Two new modified Bacillus thuringiensis (Bt) proteins, Cry1Da_7 and Cry1B.868, with activity against fall armyworms (FAW), Spodoptera frugiperda (J.E. Smith), were evaluated for their potential to bind new insect receptors compared to proteins currently deployed as plant-incorporated protectants (PIPs) in row crops. Results from resistant insect bioassays, disabled insecticidal protein (DIP) bioassays, and cell-based assays using insect cells expressing individual receptors demonstrate that receptor utilizations of the newly modified Cry1Da_7 and Cry1B.868 proteins are distinct from each other and from those of commercially available Bt proteins such as Cry1F, Cry1A.105, Cry2Ab, and Vip3A. Accordingly, these two proteins target different insect proteins in FAW midgut cells and when pyramided together should provide durability in the field against this economically important pest. Taken together, these results support the conclusion that Cry1Da_7 and Cry1B.868 are effective insecticidal proteins against FAW that have the same pore-forming mode of action as other three-domain Bt proteins but bind to different receptors, suggesting that they would control resistance and increase product durability.

Cry1B.868 was developed using chimeragenesis, similar to the method used to develop the Cry1A.105 protein, a familiar protein that has been deployed commercially as Bt maize protected against FAW. Cry1B.868 exerted mortality and developmental delay on FAW (and other lepidopteran insects [not shown]) at concentrations between 100 and 34,500 ng/cm2. Its MIC50 of 430 ng/cm2 against FAW using gradient-purified protein suggested an 8-fold improvement in specific activity toward this insect compared to the parental Cry1Be2 protein. There was no detectable difference in insect responses between the Cry1Fa-SS and Cry1Fa-RR colonies for both Cry1Da_7 and Cry1B.868, suggesting that the Cry1F-resistant colony was not cross-resistant to either Cry1Da_7 or Cry1B.868. Cry1B.868 was also highly toxic to the FAW colonies, with LC50 values of 262 ng/cm2 against the Vip3A-SS colony and 43 ng/cm2 against the Vip3A-RR colony, indicating a lack of cross-resistance. Interestingly, the Vip3A-resistant colony was significantly more sensitive to Cry1B.868 than the Vip3A-susceptible colony was; the data suggest that this difference is unrelated to the Vip3A resistance allele, and it is likely due to slight genetic background differences between the susceptible and resistant colonies. Cry1B.868 at 50 μg/ml elicited robust membrane permeabilization in Sf9 cells expressing Sf.ABCb1, while only a background signal was observed when this receptor was not expressed. These results indicate that SfABCb1 and Cry1B.868 are a functional receptor-toxin pair.

> IEDSLCIAEGNNIDPFVSASTVQTGINIAGRILGVLGVPFAGQIASFYSFLVGELWPRGRDPWEIFLEHVEQLIRQQVTENTRDTALARLQGLGNSFRAYQQSLEDWLENRDDARTRSVLYTQYINLELDFLDAMPLFAIRNQEVPLLMVYAQAANLHLLLLRDASLFGSEFGLTSQEIQRYYERQVEKTREYSDYCARWYNTGLNNLRGTNAESWLRYNQFRRDLTLGVLDLVALFPSYDTRVYPMNTSAQLTREIYTDPIGRTNAPSGFASTNWFNNNAPSFSAIEAAVIRPPHLLDFPEQLTIFSVLSRWSNTQYMNYWVGHRLESRTIRGSLSTSTHGNTNTSINPVTLQFTSRDVYRTESFAGINILLTTPVNGVPWARFNWRNPLNSLRGSLLYTIGYTGVGTQLFDSETELPPETTERPNYESYSHRLSNIRLISGNTLRAPVYSWTHRSADRTNTISSDSITQIPLVKAHTLQSGTTVVKGPGFTGGDILRRTSGGPFAFSNVNLDFNLSQRYRARIRYASTTNLRIYVTVAGERIFAGQFDKTMDAGAPLTFQSFSYATINTAFTFPERSSSLTVGADTFSSGNEVYVDRFELIPVTATFEAESDLER> QEHEPIGAQDERLSTLIHQRMQEAKVPALSVSVTIKG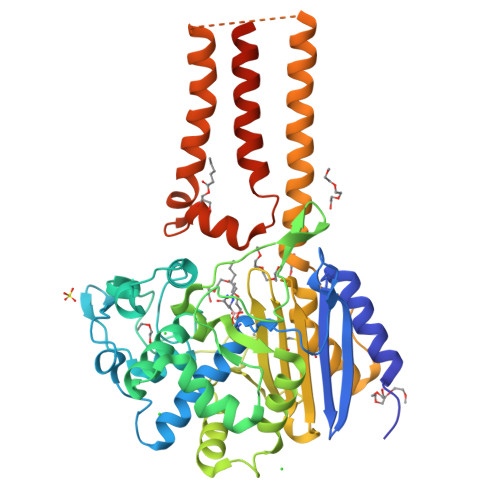VRQRFVYGVADVASQKANTLDTVYELGSMSKAFTGLVVQILIQEGRLRQGDDIITYLPEMRLNYQGKPASLTVADFLYHTSGLPFSTLARLENPMPGSAVAQQLRNENLLFAPGAKFSYASANYDVLGAVIENVTGKTFTEVIAERLTQPLGMSATVAVKGDEIIVNKASGYKLGFGKPVLFHAPLARNHVPAAYIHSTLPDMEIWIDAWLHRKALPATLREAMSNSWRGNSDVPLAADNRILYASGWFIDQNQGPYISHGGQNPNFSSCIALRPDQQIGIVALANMNSNLILQLCADIDNYLRIGKYADGAGDAITATDTLFVYLTLLLCFWGAVVVVRGAFRVYRATAHGPGKQQRLRLRVRDYIIALAVPGLVAAMLYVAPGILSPGLDWRFILVWGPSSVLAIPFGIILLAFVLTLNHQIKRILLHNKEWDDEHHHHHH>MGSSHHHHHHSSGLVPRGSHMKEAGQMQNLESARAGRSVSTQTGSMTGQIPRLSKVNLFTLLSLWMELFPAEAQRQKSQKNEEGKHGPLGDNEERTRVSTDKRQVKRTGLVVVKNMKIVGLHCSSEDLHAGQIALIKHGSRLKNCDLYFSRKPCSACLKMIVNAGVNRISYWPADPEISLLTEASSSEDAKLDAKAVERLKSNSRAHVCVLLQPLVCYMVQFVEETSYKCDFIQKITKTLPDANTDFYYECKQERIKEYEMLFLVSNEEMHKQILMTIGLENLCENPYFSNLRQNMKDLILLLATVASSVPNFKHFGFYRSNPEQINEIHNQSLPQEIARHCMVQARLLAYRTEDHKTGVGAVIWAEGKSRSCDGTGAMYFVGCGYNAFPVGSEYADFPHMDDKQKDREIRKFRYIIHAAQNALTFRCQEIKPEERSMIFVTKCPCDECVPLIKGAGIKQIYAGDVDVGKKKADISYMRFGELEGVSKFTWQLNPSGAYGLEQNEPERRENGVLRPVPQKEEQHQDKKLRLGIH[6x]

Vertebrates possess a second DCTD-like protein, CDADC1 (NYD-SP15). Unlike DCTD, CDADC1 contains two CMP/dCMP-like deaminase domains (IPR002125), connected by a long (>100 residues) linker within a single polypeptide chain, resulting in CDADC1 being approximately triple the length of DCTD (e.g. 514 residues in human CDADC1 versus 178 in human DCTD). The C-terminal deaminase domain (CTD) of CDADC1 contains a potentially active HAE motif, but its N-terminal domain (NTD) appears to be naturally inactivated due to the mutation of the proton shuttle glutamate (the HAG motif instead of HAE), suggesting noncatalytic function. In this work, we provide biochemical and structural evidence that human CDADC1 deaminates dCTP and CTP.

In the presence of dCTP, each CDADC1 protomer contains a well-defined dCTP in the active site, therefore one CDADC1 hexamer binds six dCTP molecules. Within the active site, the cytosine base of dCTP stacks under Zn2+ coordinating H398. In the absence of E400, dCTP N4 displaces the Zn2+ bound water molecule of the ligand-free structures and participates in the Zn2+ coordination, mimicking the transition state. The C5 of dCTP is located at <4 Å from C426, I455, and Y457, strongly suggesting that the low CDADC1 activity on 5mdCTP and 5hmdCTP is a result of a steric conflict. Accommodation of dCTP also drives the significant rearrangement of the K392-F393 region, likely due to the steric conflict between the 3′OH and α-phosphate (αP) on the dCTP side and aromatic ring of the F393 on the CDADC1 side. Astonishingly, five lysine residues that constitute the positively charged patch on the CDADC1 surface all rearrange to form salt bridges with dCTP phosphates. The incorporation of dCTP into the active site triggers a cascade of structural changes on an increasing scale. The loop region between these two threonines undergoes reorganization to avoid the collision between K393 and K377 bound to dCTP and H336. All the above leads to the stabilization of a large unstructured region (residues 376–390). Most importantly, the two antiparallel protomers that are too far from each other to form contacts in the absence of substrate, directly interact in the presence of dCTP. Upon dCTP binding, the combined interface area in CDADC1 hexamer increases to ~1,130 Å2 per protomer.> SASNYPAYMDNYLKEVINQVEQETGYNLLTTGMDVYTNVDQEAQKHLWDIYNSDQYVSYPDDDLQVASTVVDVSNGKVIAQLGARHQASNVSFGTNQAVETNRDWGSAMKPITDY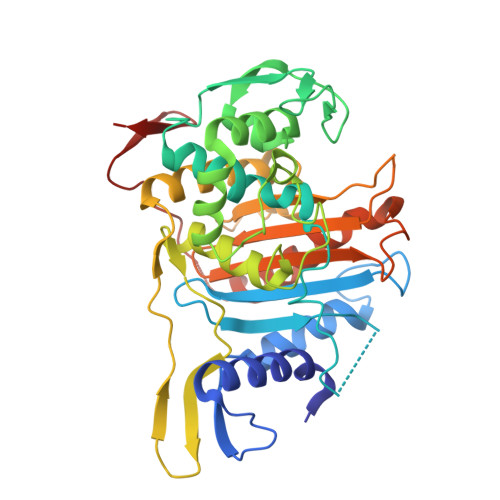APAIEYGVYDSTATMVNDIPYNYPGTSTPVYNWDRAYFGNITLQYALQQSRNVTAVETLNKVGLDRAKTFLNGLGIDYPSMHYANAISSNTTESNKQYGASSEKMAAAYAAFANGGIYHKPMYINKVVFSDGSKKEFSDVGTRAMKETTAYMMTEMMKTVLAYGTGRGAYLPWLAQAGKTGTSNYTDDEIEKHIKNTGYVAPDEMFVGYTRKYSMAVWTGYSNRLTPIVGDGFLVAAKVYRSMITYLSEGSNPEDWNIPEGLYRNGEFVFKNGAR Whereas previous studies on salivary gland extracts from the sandfly Lutzomyia longipalpis identified SALO (salivary anticomplement from L. longipalpis) as a potent inhibitor of the classical complement pathway (CP), its precise mechanism of action has remained elusive. We found that SALO inhibits the CP by binding specifically to the zymogen form of C1r. We provide two crystal structure determinations and supporting functional studies which show that SALO binds tightly to the zymogen activation loop of C1r preventing cleavage of its scissile bond. However, since the C1r zymogen undergoes autoactivation over time, we expressed an engineered fragment of human C1r consisting of its two CCP repeats and its serine protease domain, wherein the catalytic serine (S654) had been mutated to alanine (zC1r-12SP).

To further investigate this modification, we crystallized the eSALO-Y51F mutant with zC1r-12SP, collected X-ray diffraction data extending to 3.1 Å limiting resolution, and solved the structure by molecular replacement. After completing model building and refinement, our final model had Rwork and Rfree values of 23.1% and 27.8%, respectively. We found that the eSALO-Y51F–zC1r-12SP structure largely mirrored that of eSALO-WT–zC1r-12SP. Although the contributions from the sulfate modification were expectedly absent, many of the interactions present in the WT structure were maintained. This included the hydrogen bonds formed by D32 and the salt bridges formed by E58 but not the hydrogen bonds formed by N33. Overall, these structures showed that sulfation of SALO Y51 promoted interactions with residues sharing the scissile bond of the C1r zymogen, but that sulfation was not necessary for SALO binding to the C1r zymogen. However, we found that the affinity of eSALO-Y51F for C1r proenzyme and zC1r-12SP was diminished 7.5-fold and 8.2-fold, respectively. We found that eSALO-E58A displayed an IC50 value diminished by 14.1-fold, whereas eSALO-Y51F was even less potent with an estimated 171-fold loss compared with eSALO-WT. At the functional level, this modification appeared to result in an ∼8-fold gain in affinity for the C1r zymogen and an ∼170-fold gain in potency in CP-dependent hemolytic assays, as judged by comparison of eSALO-WT and eSALO-Y51F.

>[2x]SEDCENIFHDNAYLLKLDCEAGRVDPVEFDDISDEEIYEITVDVGVSSEDQEKVAKIIRECIAQVSTQDCTKFSEIYDCYMKKKICNYYPENMGSGHHHHHHHH;>[2x]KCPQPKTLDEFTIIQNLQPQYQFRDYFIATCKQGYQLIEGNQVLHSFTAVCQDDGTWHRAMPRCKIKDCGQPRNLPNGDFRYTTTMGVNTYKARIQYYCHEPYYKMQTRAGSRESEQGVYTCTAQGIWKNEQKGEKIPRCLPVCGKPVNPVEQRQRIIGGQKAKMGNFPWQVFTNIHGRGGGALLGDRWILTAAHTLYPKEHEAQSNASLDVFLGHTNVEELMKLGNHPIRRVSVHPDYRQDESYNFEGDIALLELENSVTLGPNLLPICLPDNDTFYDLGLMGYVSGFGVMEEKIAHDLRFVRLPVANPQACENWLRGKNRMDVFSQNMFCAGHPSLKQDACQGDAGGVFAVRDPNTDRWVATGIVSWGIGCSRGYGFYTKVLNYVDWIKKEMEEEDGSGHHHHHHHH>[2x]EVRLSVPPLVEVMRGKSVILDCTPTGTHDHYMLEWFLTDRSGARPRLASAEMQGSELQVTMHDTRGRSPPYQLDSQGRLVLAEAQVGDERDYVCVVRAGAAGTA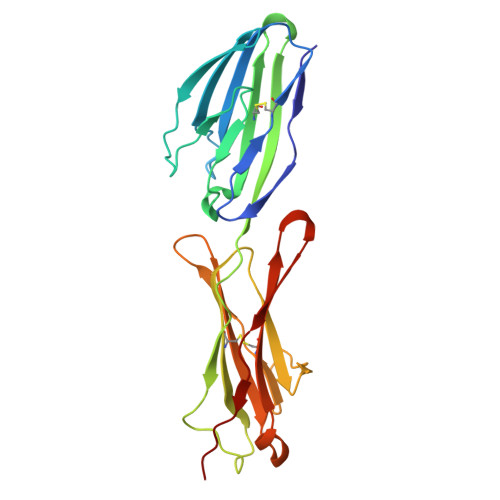EATARLNVFAKPEATEVSPNKGTLSVMEDSAQEIATCNSRNGNPAPKITWYRNGQRLEVPVEMNPEGYMTSRTVREASGLLSLTSTLYLRLRKDDRDASFHCAAHYSLPEGRHGRLDSPTFHLTLHY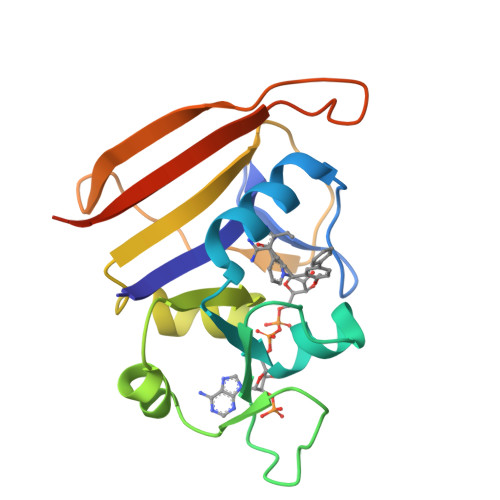>TLSILVAHDLQRVIGFENQLPWHLPNDLKHVKKLSTGHTLVMGRKTFESIGKPLPNRRNVVLTSDTSFNVEGVDVIHSIEDIYQLPGHVFIFGGQTLFEEMIDKVDDMYITVIEGKFRGDTFFPPYTFEDWEVASSVEGKLDEKNTIPHTFLHLIRKLEHHHHHHHH[2x]>MASQGPGEVVLLDFAAAGGELGWLTHPYGKGWDLMQNIMNDMPIYMYSVCNVMSGDQDNWLRTNWVYRGEAERIFIELKFTVRDCNSFPGGASSCKETFNLYYAESDLDYGTNFQKRLFTKIDTIAPDEITVSSDFEARHVKLNVEERSVGPLTRKGFYLAFQDIGACV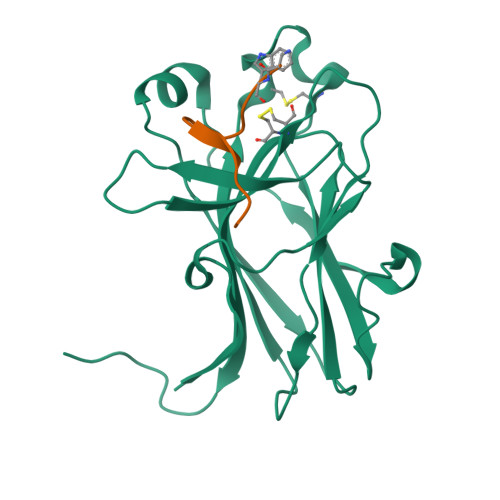ALLSVRVYYKKAHHHHHH[2x];>[2x]XWLAYPDSVPYRPK>MHHHHHHEENVKRRTHNVLERQRRNELKRSFFALRDQIPELENNEKAPKVVILKKATAYILSVQAEEQKLISEEDLLRKRREQLKHKLEQLRNS[4x];>MADKRAHHNALERKRRDHIKDSFHSLRDSVPSLQGEK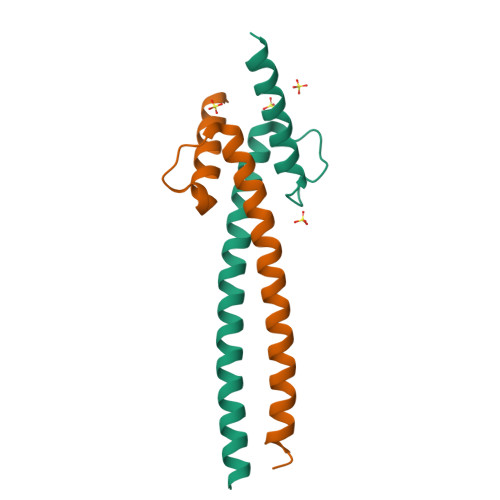ASRAQILDKATEYIQYMRRKNHTHQQDIDDLKRQNALLEQQVRALE[4x]>MRGETLKLKKDKRREAIRQQIDSNPFITDHELSDLFQVSIQTIRLDRTYLNIPELRKRIKLVAEKNYDQISSIEEQEFIGDLIQVNPNVKAQSILDITSDSVFHKTGIARGHVLFAQANSLCVALIKQPTVLTHESSIQFIEKVKLNDTVRAEARVVNQTAKHYYVEVKSYVKH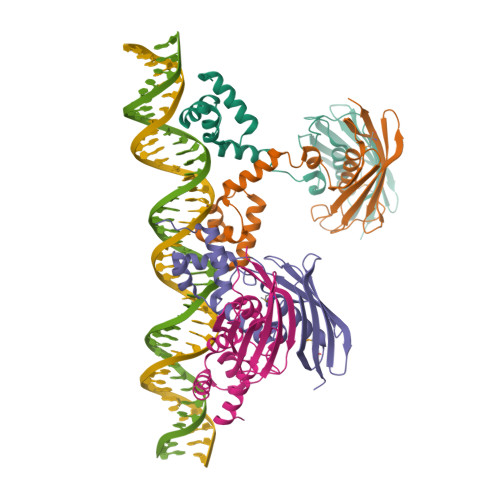TLVFKGNFKMFYDKRG[4x]>MSNEIP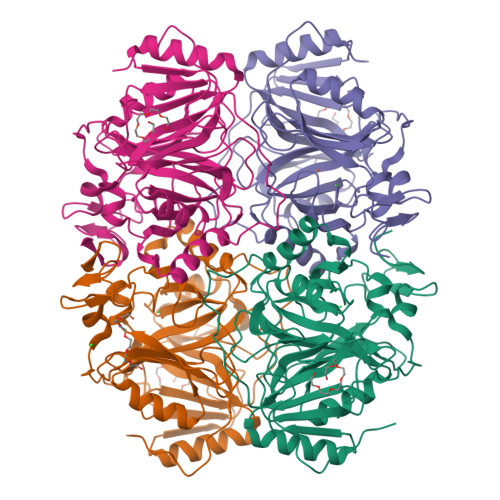KPVAPAPDILRCAYAELVVTDLAKSRNFYVDVLGLHVSYEDENQIYLRSFEEFIHHNLVLTKGPVAALKAMAFRVRTPEDVDKAEAYYQELGCRTERRKDGFVKGIGDALRVEDPLGFPYEFFFETTHVERLHMRYDLYSAGELVRLDHFNQVTPDVPRGRKYLEDLGFRVTEDIQDDEGTTYAAWMHRKGTVNDTALTGGNGPRLHHVAFSTHEKHNIIQICDKMGALRISDRIERGPGRHGVSNAFYLYILDPDNHRIEIYTQDYYTGDPDNPTITWNVHDNQRRDWWGNPVVPSWYTEASKVLDLDGNVQEIIERTDDSELEVTIGADGFSFTRAGDEDGSYHGQASKGFKLGNQL[4x]>[2x]SNAEPPTNLDKPEGRLDIIAWPGYIERGQTDKQYDWVTQFEKETGCAVNVKTAA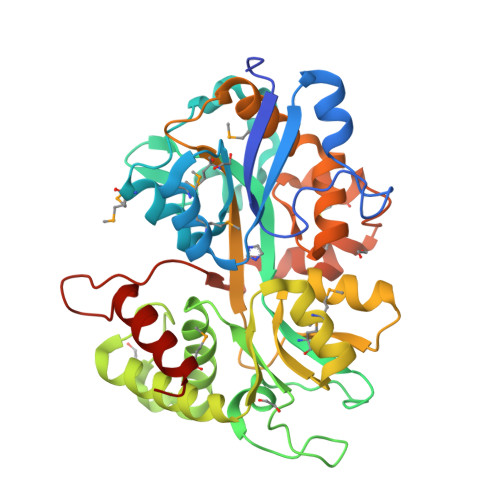TSDEMVSLMTKGGYDLVTASGDASLRLIMGKRVQPINTALIPNWKTLDPRVVKGDWFNVGGKVYGTPYQWGPNLLMYNTKTFPTPPDSWQVVFVEQNLPDGKSNKGRVQAYDGPIYIADAALFVKATQPQLGISDPYQLTEEQYQAVLKVLRAQHSLIHRYWHDTTVQMSDFKNEGVVASSAWPYQANALKAEGQPVATVFPKEGVTGWADTTMLHSEAKHPVCAYKWMNWSLTPKVQGDVAAWFGSLPVVPEGCKASPLLGEKGCETNGFNYFDKIAFWKTPIAEGGKFVPYSRWTQDYIAIMGGR> MAVLKGLRPRVPKGLKSPPEPWGWPLLGHVLTLGKNPHLALSRMSQRYGDVLQIRIGSTPVLVLSRLDTIRQALVRQGDDFKGRPDLYTSTLITDGQSLTFSTDSGPVWAARRRLAQNALNTFSIASDPASSSSCYLEEHVSKEAKALISRLQELMAGPGHFDPYNQVVVSVANVIGAMCFGQHFPESSDEMLSLVKNTHEFVETASSGNPLDFFPILRYLPNPALQRFKAFNQRFLW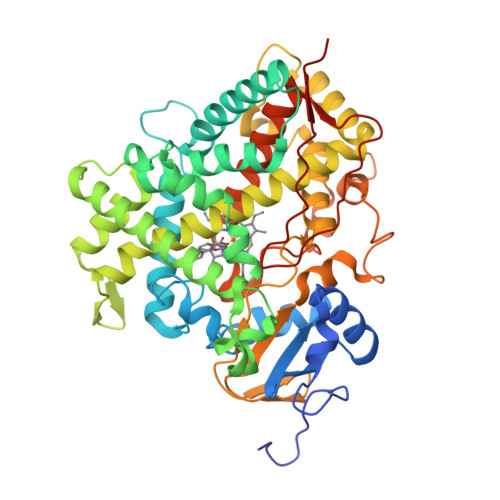FLQKTVQEHYQDFDKNSVRDITGALFKHSKKGPRASGNLIPQEKIVNLVNDIFGAGFDTVTTAISWSLMYLVTKPEIQRKIQKELDTVIGRERRPRLSDRPQLPYLEAFILETFRHSSFLPFTIPHSTTRDTTLNGFYIPKKCCVFVNQWQVNHDPELWEDPSEFRPERFLTADGTAINKPLSEKMMLFGMGKRRCIGEVLAKWEIFLFLAILLQQLEFSVPPGVKVDLTPIYGLTMKHARCEHVQARRFSINHHHH>[3x]AMGYLMALFEDIQAVIAEQLNVDAAQVTPEAEFVKDLGAD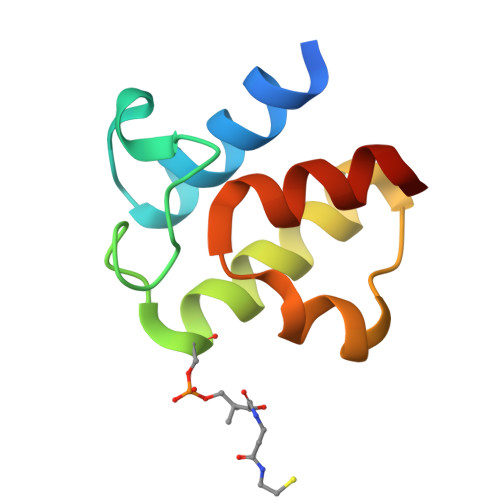XLDVVELIMALEEKFGIEIPDEQAEKIVNVGDVVKYIEDNKLA>[2x]GADPKKVLDQAKDQMENVVR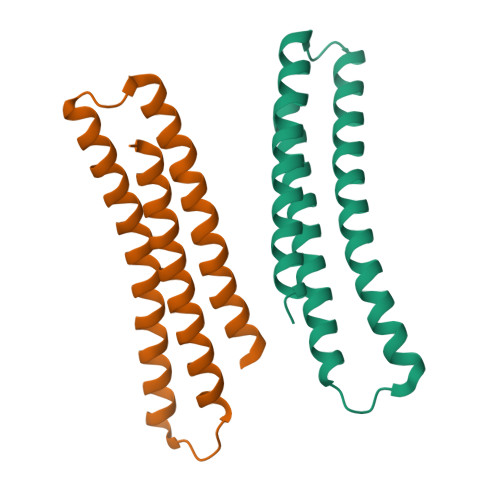TLKQELEELAKEARKLDLTQSEKIELKLRYIVAHLAAIGDIEEAIREAKEEADKLKRAGLVNSQQFDEFKRRLEELHKEADRKRADYAEEFRNKLEYG> SVQQASRSKVSVAPLHLESAKEPPLNTYKPKEPFTATIVSVESLVGPKAPGETCHIVIDHGGNVPYWEGQSYGVIPPGENPKKPGAPQNVRLYSIASTRYGDNFDGRTGSLCVRRAVYYDPETGKEDPSKNGVCSNFLCNSKPGDKIQLTGPSGKIMLLPEEDPNATHIMIATGTGVAPFRGYLRRMFMEDVPNYRFGGLAWLFLGVANSDSLLYDEEFTSYLKQYPDNFRYDKALSREQKNRSGGKMYVQDKIEEYSDEIFKLLDGGAHIYFCG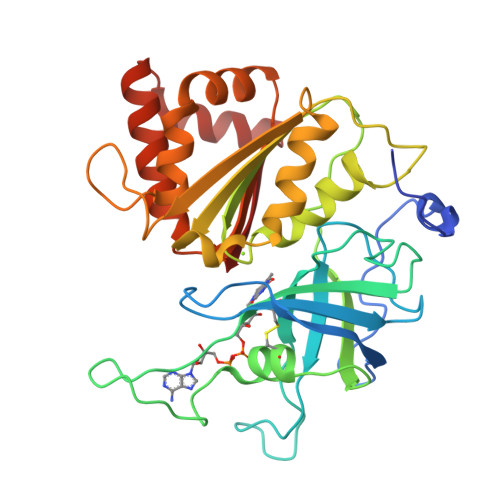LKGMMPGIQDTLKKVAERRGESWDQKLAQLKKNKQWHVEVF>GALPSHNKASFTDEEDEFILDVVRKNPTRRTTHTLYDEISHYVPNHTGNSIRHRFRVYLSKRLEYVYEVDKFGKLVRDDDGNLIKTKVLPPSIKRKFSADEDYTLAIAVKKQFYRDLFQIDPDTGRSLITDEDTPTAIARRNMTM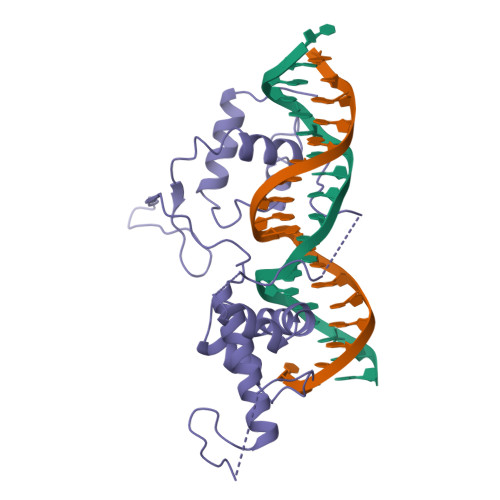DPNHVPGSEPNFAAYRTQSRRGPIAREFFKHFAEEHAAHTENAWRDRFRKFLLAYGIDDYISYYEAEKAQNREPEPMKNLTNRPKRPGVPTPGNYNSAAKR[2x]>[2x]MMNDGKQQSTFLFHDYETFGTHPALDRPAQFAAIRTDSEFNVIGEPEVFYCKPADDYLPQPGAVLITGITPQEARAKGENEAAFA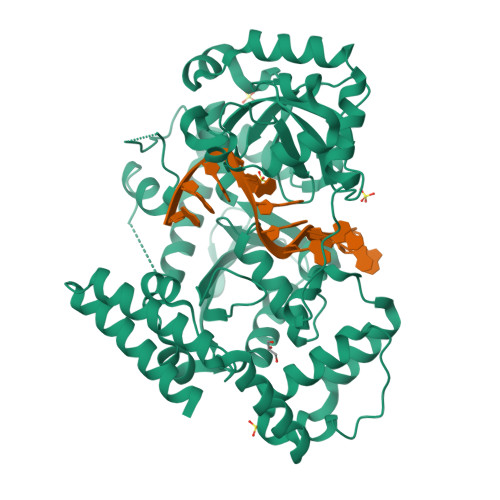ARIHSLFTVPKTCILGYNNVRFDDEVTRNIFYRNFYDPYAWSWQHDNSRWDLLDVMRACYALRPEGINWPENDDGLPSFRLEHLTKANGIEHSNAHDAMADVYATIAMAKLVKTRQPRLFDYLFTHRNKHKLMALIDVPQMKPLVHVSGMFGAWRGNTSWVAPLAWHPENRNAVIMVDLAGDISPLLELDSDTLRERLYTAKTDLGDNAAVPVKLVHINKCPVLAQANTLRPEDADRLGINRQHCLDNLKILRENPQVREKVVAIFAEAEPFTPSDNVDAQLYNGFFSDADRAAMKIVLETEPRNLPALDITFVDKRIEKLLFNYRARNFPGTLDYAEQQRWLEHRRQVFTPEFLQGYADELQMLVQQYADDKEKVALLKALWQYADEIVHHHHHH>[4x]GSSHHHHHHSQDPNSMVSESNRGGADRTTAAGEEKEERGQLLFDVPEIRFTKLFINGSFVDAVSGR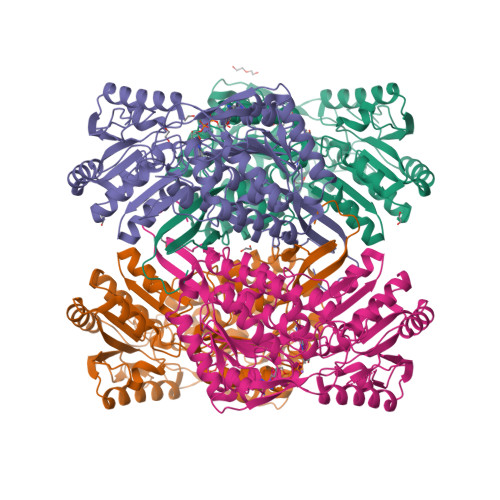TFDTRDPRTGGVIASVAEADKEDVDLAVRAARAAFDHGEWPRMSGSERGRIMARLADLVEEHAGELAALESLDAGKHPAVTRAVDVGNAAGSLRYFAGAADKIHGETLKMPGQFQGHTLREPLGVAGVIIPWNFPSTMFAVKVAPALAAGCALVVKPAEQTPLSALYLAQLAKQAGVPDGVINVVPGFGPTAGAALASHMDVDMVSFTGSTEVGRLIMKASAESNLKPVYLELGGKSPLIVFDDADLDMAVELAVGASFFNKGEACVAASRVYVQERVYDRFEERLAERMRSWVVGDPFSDPRADQGPQVDKAQYERVLSYIDHGKREGATLLTGGRPCAPEGKGYYIEPTVFTNVKEDMIIAKEEIFGPVMCLMKFKTVEEAIARANDTRYGLGAGVVTRDLDVANRVVRSVRAGVVWVNCYFAMGSDCPFGGRKMSGFGKDEGMHALDKYLAVKSVVTPLRASPWI>[4x]EGDIHMKKGHHH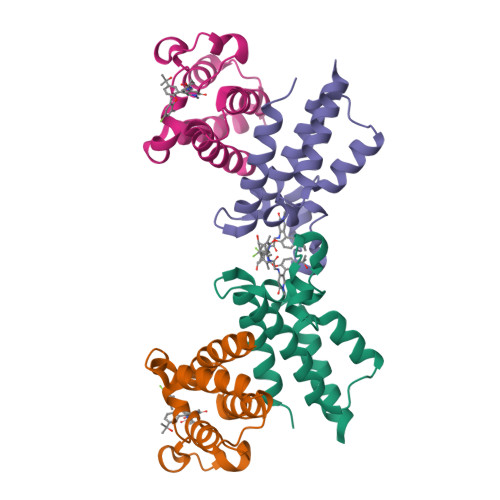HHHENLYFQGGSGKLSEQLKHCNGILKELLSKKHAAYAWPFYKPVDASALGLHDYHDIIKHPMDLSTVKRKMENRDYRDAQEFAADVRLMFSNCYKYNPPDHDVVAMARKLQDVFEFRYAKMPD(3S)-3-(dihydroxy-lambda~4~-sulfanyl)-4-(1H-1,2,3-triazol-1-yl)-D-valine 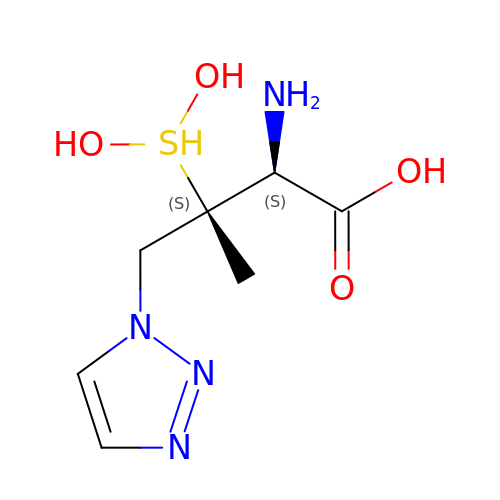| C7 H14 N4 O4 S | YZPZKAQMEJGYGB-FSPLSTOPSA-N N-phenyl-3-sulfanylpropanamide | C9 H11 N 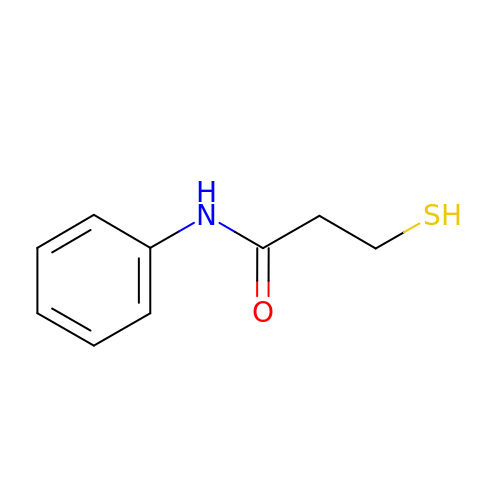O S | YSPHRFZMBKXSAX-UHFFFAOYSA-N>[4x]MKPKVVLTHWVHPEIIELLSASADVIPNTTRETLPRSEVIARAKDADALMAFMPDSIDSAFLEECPKLRVIGAALKGYDNFDVNACTRHGVWLTIVPDLLTIPTAELTIGLLLGLTRHMLEGDRQIRSGH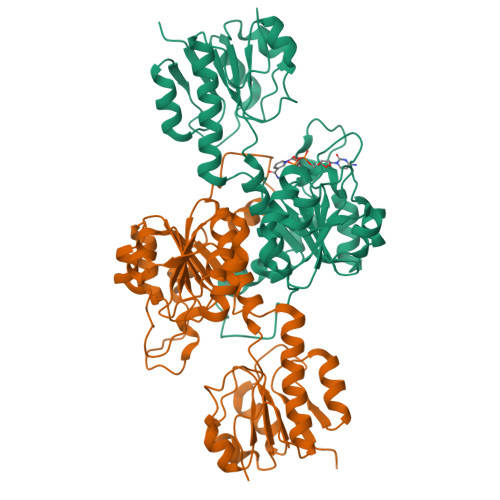FQGWRPTLYGSGLTGKTLGIRGMGAVGRAIAQRLAGFEMNLLYCDRIPLNAEQEKAWHVQRVTLDELLEKCDYVVPAVPMAAETLHLIDATALAKMKTGSYLINACRGSVVDENAVIAALASGKLAGYAADVFEMEEWIRADRPQAIPKALLDNTAQTFFTPHLGSAVKEVRLEIERQAAMNIIQALAGEKPMGAINQPYPGVKAALE> ASMQKLINSVQNYAWGSKTALTELYGIANPQQQPMAELWMGAHPKSSSRITTANGETVSLRDAIEKNKTAMLGEAVANRFGELPFLFKVLCAAQPLSIQVHPNKRNSEIGFAKENAAGIPMDAAERNYKDPNHKPALVFALTPFLAMNAFREFSDIVSLLQPVAGAHSAIAHFLQVPNAERLSQLFASLLNMQGEEKSRALAVLKAALNSQQGEPWQTIRVISEYYPDDSGLFSPLLLNVVKLNPGEAMFLFAETPHAYLQGVALEVMANSDNVLRAGLTPKYIDIPELVANVKFEPKPAGELLTAPVKSGAELDFPIPVDDFAFSLHDLALQETSIGQHSAAILFCVEGEAVLRKDEQRLVLKPGESAFIGADESPVNASGTG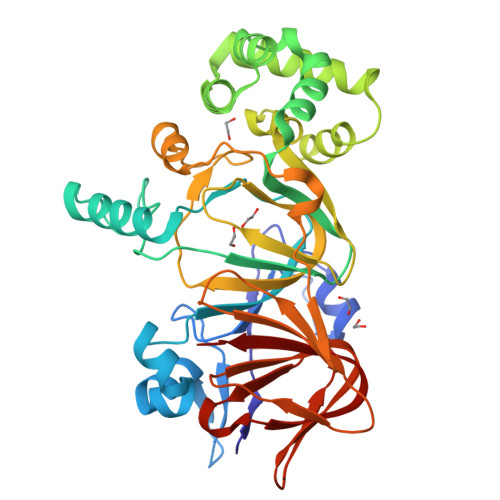RLARVYNKL> MRKSLFAVMVLALVAAFALPVIAAEAPADGLKMENTKMPVIFNHSSHSSYQCADC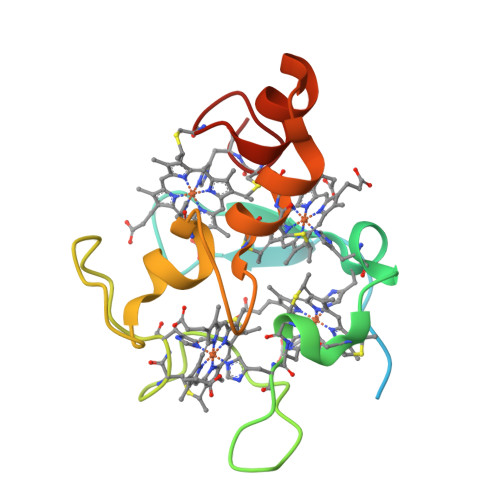HHPVDGKENLAKCATAGCHDVFDKKDKSVHSYYKIIHDRKATTVATCMSCHLEAAGSDKDLKKELTGCKKSKCHP N-[3-({4-[(3-aminopropyl)amino]-5-iodopyrimidin-2-yl}amino)phenyl]pyrrolidine-1-carboxamide | 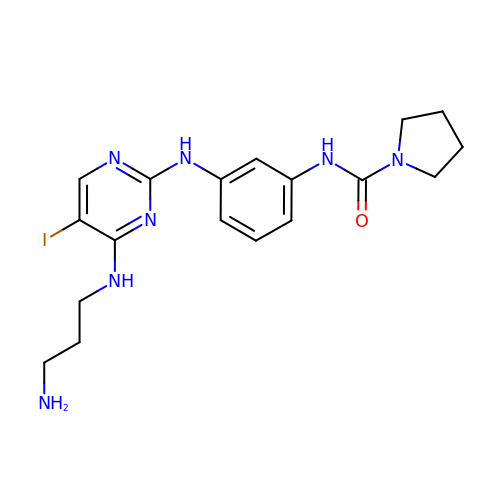C18 H24 I N7 O | ZYLHCSSOEGIFAO-UHFFFAOYSA-N>[4x]MGSSHHHHHHSAGENLYFQGQQGDLMPQSALFTGIIPPVSTIFTADGQLDKPGTAALIDDLIKAGVDGLFFLGSGGEFSQLGAEERKAIARFAIDHVDRRVPVLIGTGGTNARETIELSQHA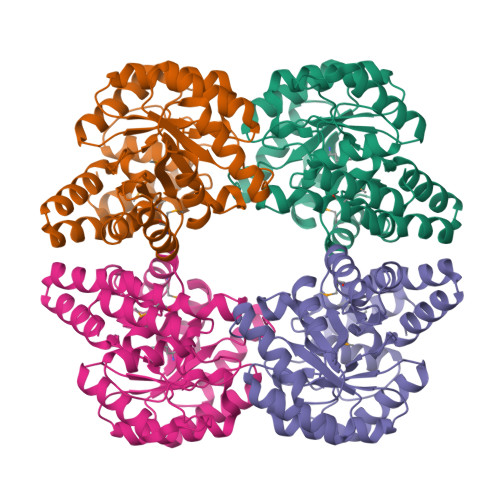QQAGADGIVVINPYYWKVSEANLIRYFEQVADSVTLPVMLYNFPALTGQDLTPALVKTLADSRSNIIGIKDTIDSVAHLRSMIHTVKGAHPHFTVLCGYDDHLFNTLLLGGDGAISASGNFAPQVSVNLLKAWRDGDVAKAAGYHQTLLQIPQMYQLDTPFVNVIKEAIVLCGRPVSTHVLPPASPLDEPRKAQLKTLLQQLKLCCGRTRAPPPPPLRSGC>[4x]HHHHHHMKGFAMLSIGKVGWIEKEKPAPGPFDAIVRPLAVAPCTSDIHTVFEGAIGERHNMILGHEAVGEVVEVGSEVKDFKPGDRVVVSALTPDWRTSEVQRGYHQHSGGMLAGWKFSNVKDGVFGEFFHVNDADMNLAHLPKEIPLEAAVMIPDMMTTGFHGAELADIELGATVAVLGIGPVGLMAVAGAKLRGAGRIIAVGSRPVCVDAAKYYGATDIVNYKDGPIESQIMNLTEGKGVDAAIIA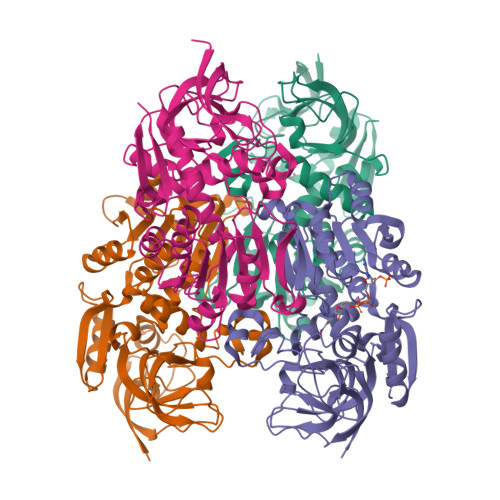GGNADIMATAVKIVKPGGTIANVNYFGEGEVLPVPRLEWGCGMAHKTIKGGLCPGGRLRMERLIDLVFYKRVDPSKLVTHVFRGFDNIEKAFMLMKDKPKDLIKPVVILA> MSKESVRNDRNKKKKEVPKPECSESYTLTPEVGELIEKVRKAHQETFPALCQLGKYTTNNSSEQRVSLDIDLWDKFSELSTKCIIKTVEFAKQLPGFTTLTIADQITLLKAACLDILILRICTRYTPEQDTMTFSDGLTLNRTQMHNAGFGPLTDLVFAFANQLLPLEMDDAETGLLSAICLICGDRQDLEQPDRVDMLQEPLLEALKVYVRKRRPSRPHMFPKMLMKITDLRSISAKGAERVITLK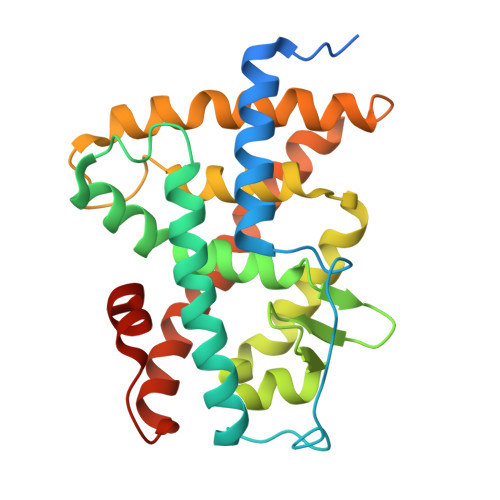MEIPGSMPPLIQEMLENSEGLD>HHHHHHKVDLGGFAGLFDLKAAGFKDPLLASGTDGVGTKLKIAQLCNKHDTIGQDLVAMCVNDILAQGAEPLFFLDYFSCGKLDLSVTEAVVAGIAKACGKAGCALLGGETAEMPDMYPPGEYDLAGFAVGAMERDQKLPHLERITEGDVVVGIASSGLHSNGFSLVRKIVAKSSLQYSSPAPDGCGDQTLGDLLLTPTRIYSHSLLPVLRSGHVKAFAHITGGGLLENIPRVLPEKLGVDLDAQTWRIPRVFSWLQQEGHLSEEEMARTFNCG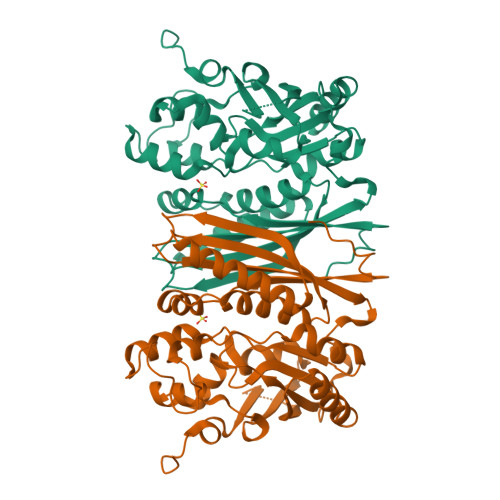VGAVLVVSKEQTEQILRGIQQHKEEAWVIGSVVARAEGSPRVKVKNLIESMQINGSVLKN[2x]HIT is caused by antibodies to complexes that form between platelet factor 4 (PF4) released from activated platelets and heparin or cellular glycosaminoglycans (GAGs). Here we describe and compare the crystal structures of PF4 in complex with Fabs derived from KKO and RTO and the structure of PF4 in complex with a heparin-mimic pentasaccharide, fondaparinux. NMR studies reveal that PF4 exists as an equilibrium among monomers, dimers and tetramers. Each monomer contains three-stranded antiparallel β-sheets on which an aperiodic N-terminal domain and an amphipathic C-terminal α-helix are folded.

To investigate how the GAGs might induce or augment neoantigen formation, we crystallized PF4 in complex with fondaparinux, a homogenous synthetic pentasaccharide heparin that forms complexes with PF4 as assessed by atomic force microscopy and photon correlation spectroscopy. We solved the crystal structure of PF4 in complex with fondaparinux as a model GAG. The PF4/fondaparinux complex is a pseudo-222 tetramer formed by a pseudo two-fold non-crystallographic symmetry and a perpendicular two-fold crystallographic symmetry (Table 1 for statistics). Fondaparinux appears as a well-defined molecule, evidenced by the strong and clear electron densities. The PF4 tetramer displays a pseudosymmetry characterized by an ‘open' end and a ‘closed' end that can be defined by the intra-chain distances between amino acids E28 and K50. E28 and K50 are ∼3 Å apart and form stable salt bridge pairs between chain A and chain C. However, the same interchain salt bridge pairs do not form between E28 and K50 in chains B and D, which are ∼8 Å apart. This asymmetry in the PF4 tetramer explains why calculation of its electrostatic potential identifies only two positively charged grooves on the ‘closed' side of PF4 tetramer surface to which fondaparinux can bind. Fondaparinux binds among monomers A, B and C or monomers A, C and D. This interaction stabilizes the AB/CD association and the AC/BD association, thus further stabilizing the PF4 tetramer. One fondaparinux molecule not only binds within the groove on the surface of one PF4 tetramer, it is also shared with a second symmetry-related tetramer through binding to its C-terminal helix.

>[2x]EAEEDGDLQCLCVKTTSQVRPRHITSLEVIKAGPHCPTAQLIATLKNGRKICLDLQAPLYKKIIKKLLES>MYNYKEVKHMGYGKGYLAMFKNKKVRFKVVNSFPDLKVQFVTSFPDYKVKISNSSSFCEETIKIQVVTSFPD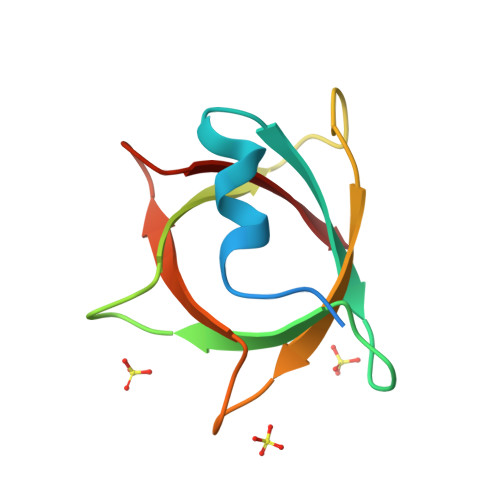VKLQKVTSFGDFEAYID[8x]> MYNGKDRAQNSYQPMYQRPMQVQGQQQAQSFVGKKNTIGSVHGKAPMLMANNDVFTIGPYRARKDRMRVSVLEKYEVIGYIAAGTYGKVYKAKRQINSGTNSANGSSLNGTNAKIPQFDSTQPKSSSSMDMQANTNALRRNLLKDEGVTPGRIRTTREDVSPHYNSQKQTLIKKPLTVFYAIKKFKTEKDGVEQLHYTGISQSACREMALCRELHNKHLTTLVEIFLERKCVHMVYEYAEHDLLQIIHFHSHPEKRMIPPRMVRSIMWQLLDGVSYLHQNWVLHRDLKPANIMVTIDGCVKIGDLGLARKFHNMLQTLYTGDKVVVTIWYRAPELLLGARHYTPAVDLWSVGCIFAELIGLQPIFKGEEAKLDSKKTVPFQVNQLQRILEVLGTPDQKIWPYLEKYPEYDQITKFPKYRDNLATWYHSAGGRDKHALSLLYHLLNYDPIKRIDAFNALEHKYFTESDIPVSENVFEGLTYKYPARRIHTNDNDIMNLGSRTKNNTQASGITAGAAANALGGLGVNRRILAAAAAAAAAVSGNNASDEPSRKKNRR;> MSGSFWTSTQRHHWQYTKASLAKERQKLWLLECQLFPQGLNIVMDSKQNGIEQSITKNIPITHRDLHYDKDYNLRIYCYFLIMKLGRRLNIRQYALATAHIYLSRFLIKASVREINLYMLVTTCVYLACKVEECPQYIRTLVSEARTLWPE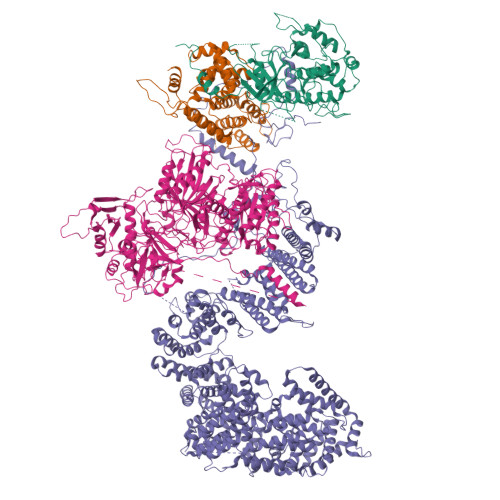FIPPDPTKVTEFEFYLLEELESYLIVHHPYQSLKQIVQVLKQPPFQITLSSDDLQNCWSLINDSYINDVHLLYPPHIIAVACLFITISIHGKPTKGSSLASAASEAIRDPKNSSSPVQIAFNRFMAESLVDLEEVMDTIQEQITLYDHWDKYHEQWIKFLLHTLYLRPASAISMEKRRWKKNFIAVSAANRFKKISSSGAL;> MNNGSGRYLLTPPDDLHPYVPSSKPQEQVYPDFKPWEHTAAEDQILANFVAKGFYHTPMVNFESISARSSVHESLVTQSNILSQQFDKIIKIREDHINKIPSNSTTTLHGPGFQLPNRITLTDHRKETWLHELSSSHTSLVKIGKFIPHGLKRRQVIEQCYLKFIPLKRAIWLIKCCYFIEWKSNHKKKRSNAAGADDAISMHLLKDWTDTFVYILEKLIFDMTNHYNDSQQLRTWKRQISYFLKLLGNCYSLRLINKEIFHHWLVEFINKMENFEFLPLSLHILMIFWNDICQIDTNAPVAATITSSQKEPFFLVTKITDMLLHKYYIVSSSKSMINDENYIINDIKKNNKIKLNILKILSSLILKIFQEQSLEVFIFPTSNWEIYKPLLFEIVSNADTNQNSDMKKKLELISYRNESLKNNSSIRNVIMSASNANDFQLTIVTCKQFPKLSCIQLNCIDTQFTKLLDDNPTEFDWPTYVDQNPLTMHKIIQLILWSIHPSRQFDHYESNQLVAKLLLLRINSTDEDLHEFQIEDAIWSLVFQLAKNFSAQKRVVSYMMPSLYRLLNILITYGIIKVPTYIRKLISSGLLYLQDSNDKFVHVQLLINLKISPLMKSQYNMVLRNVMEYDVKFYEIFNFDQLVEITEQIKMRILSNDITNLQLSKTPLSIKIMVAEWYLSHLCSGILSSVNRTVLLKIFKIFCIDLEVFHHFFKWIEFIVYHQLLSDIESLEALMDILLCYQKLFSQFINDHILFTKTFIFIYKKVLKEKDVPAYNVTSFMPFWKFFMKNFPFVLKVDNDLRIELQSVYNDEKLKTEKLKNDKSEVLKVYSMINNSNQAVGQTWNFPEVFQVNIRFLLHNSEIIDTNTSKQFQKARNNVMLLIATNLKEYNKFMSIFLKRKDFTNKNLIQLISLKLLTFEVTQNVLGLEYIIRLLPINLENNDGSYGLFLKYHKEQFIKSNFEKILLTCYELEKKYHGNECEINYYEILLKILITYGSSPKLLATSTKIIMLLLNDSVENSSNILEDILYYSTCPSETDLNDIPLGSGQPDNDTVVTNDDKSDDDDHTVDEIDHVEYYVMMDFANLWVFQAFTCFCIKKIMENNEPAMAMEDLKNFIFQIIEITNSNDLCSQIFDQLKDMQTIEMITQIVEKDFCTSCLQNNNQKIDDNYIVVVIEIITSLSMRFQRETSGMIVISMENYHLLIKIIRQLSELNEGNLSKREIQIDAVLKIFSFHQDSIFQRIIADLSADKPTSPFIDSICKLFDKISFNLRLKLFLYEILSSLKSFAIYSSTIDAPAFHTSGKVELPKKLLNLPPFQVSSFVKETKLHSGDYGEEEDADQEESFSLNLGIGIVEIAHENEQKWLIYDKKDHKYVCTFSMEPYHFISNYNTKYTDDMATGSNDTTAFNDSCVNLSLFDARFERKNPH;> MSSDASTYRLEDVLSSFYRVEKIKKINYHQYISKAQNDQWSIQMEFMLRKQDPKTLVALLSRDLWCFSINDDPVPTPPAIEHKPVSPDKIGTFTADYSKPNLPPHYALFLKALRRKIYINLALGSHNKLIQFGNACISLSGVPNYLVQLEPHLFVNGDLTVSLCAKNMGLVPMKEENLEESFLSKHALYLAPSGIRMHLAPASKQGYLITPPKHTELLLTTLSVSHGINLQNKKNLKWVAVVPDLGHLNGHTPTIASYLTPLLEAKKLVWPLHLIFAQPVADIENSTSGDPSEFHCLQDALDAIDDFIQLKQTAAYRTPGSSGVLSSNIAGTNPLSSDGAYTEQFQHYKNNSISSQPASYHSVQETNKISPKDFSPNFTGIDKLMLSPSDQFAPAFLNTPNNNINENELFNDRKQTTVSNDLENSPLKTELEANGRSLEKVNNSVSKTGSVDTLHNKEGTLEQREQNENLPSDKSDSMVDKELFGEDEDEDLFGDSNKSNSTNESNKSISDEITEDMFEMSDEEENNNNKSINKNNKEMHTDLGKDIPFFPSSEKPNIRTMSGTTKRLNGKRKYLDIPIDEMTLPTSPLYMDPGAPLPVETPRDRRKSVFAPLNFNPIIENNVDNKYKSGGKFSFSPLQKEEALNFDISMADLSSSEEEEDEEENGSSDEDLKSLNVRDDMKPSDNISTNTNIHEPQYINYSSIPSLQDSIIKQENFNSVNDANITSNKEGFNSIWKIPQNDIPQTESPLKTVDSSIQPIESNIKMTLEDNNVTSNPSEFTPNMVNSEISNLPKDKSGIPEFTPADPNLSFESSSSLPFLLRHMPLASIPDIFITPTPVVTISEKEQDILDLIAEQVVTDYNILGNLGIPKIAYRGVKDCQEGLITTTMLQLFSTFDRLNGNDTISKFYNMKQPYVFVKKHHELIKVKHDSQPFIKFLNFRPPNGIKNFKSLLLSSSFKEDCLSFAPTLSQTYINQELGFCELLKLTNEDPPGLMYLKAFDKNKLLLLAAQIVSYCSNNKNSIKNVPPILIILPLDNATLTELVDKANIFQVIKNEVCAKMPNIELYLKVIPMDFIRNVLVTVDQYVNVAISIYNMLPPKSVKFTHIAHTLPEKVNFRTMQQQQMQQQQQQQQQQQNNSTGSSSIIYYDSYIHLAYSRSVDKEWVFAALSDSYGQGSMTKTWYVGNSRGKFDDACNQIWNIALNLASKKFGKICLILTRLNGILPDDELMNWRRLSGRNIHLAVVCVDDNSKISFIDEDKLYPSFKPIYKDTRFGGRMDMTRLYDYEIRDIDQDIHGIVFQHPFPLAHSQHRCAIRSGALIKFKKCDGDTVWDKFAVNLLNCPHSDSTQLLETILEEFRNLAALNVWYGLSDGEDGHIPWHILAVKKMMNTLVHTRVKIANTSAATVHTATSSSIILSDK> MEKEKKNVFMRTFEAISRNFSEIFAKLSPGGSARLILENPEDPFSGGLEIEAKPAGKDVKRIEAMSGGEKALTALAFVFAIQKFKPAPFYLFDEIDAHLDDANVKRVADLIKESSKESQFIVITLRDVMMANADKIIGVSMRDGVSK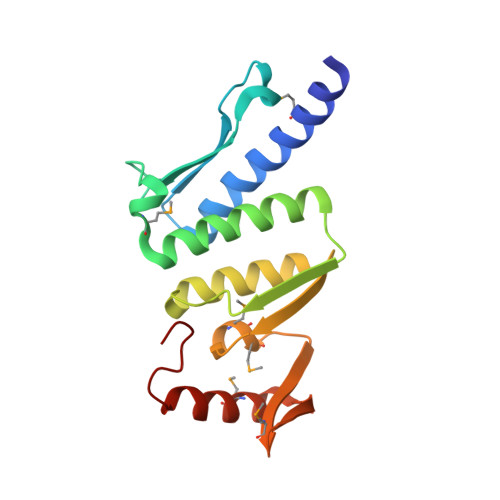VVSLSLEKAMKILEEIRKKQGWEHGN2,7-bis[3-(morpholin-4-yl)propyl]-4,9-bis{[3-(morpholin-4-yl)propyl]amino}benzo[lmn][3,8]phenanthroline-1,3,6,8(2H,7H)-tetrone | C42 H60 N8 O8 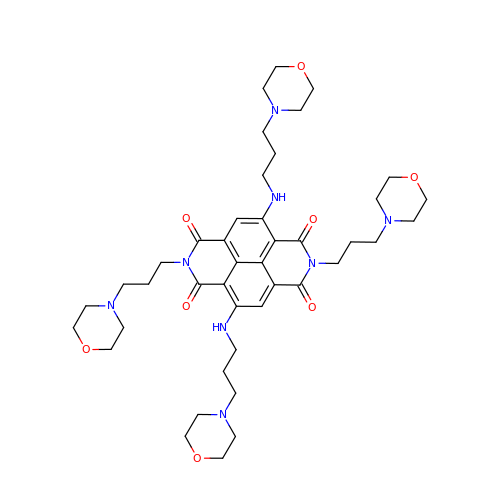| PBXBULWQEKJFOX-UHFFFAOYSA-N>[4x]MASSNVTLSNDEVLRLVKDWNFTWSVVFLLITIVLQYGYPSRSMFVYVIKMFVLWLLWPASMALSIFCAVYPIDLASQIISGILAATSCAMWISYFVQSIRLFMRTGSWWSFNPESNCLLNVPIGGTTVVRPLVEDSTSVTAVVTDGYLKMAGMHFGACDFQRLPSEVTVAKPNVLIALKMIKRQAYGTNSGVAIYHRYKAGNYRRPPIIQDQELALLRA

The membrane (M) protein is the most abundant structural protein of coronaviruses including MERS-CoV, SARS-CoV, and SARS-CoV-2, and plays a central role in virus assembly through its interaction with various partner proteins. In coronaviruses, M protein is the only multispanning transmembrane structural protein and has been shown to interact with various partner proteins, including all viral structural proteins (S, M, E, and N) and some host factors involved in the interferon signaling pathway such as MAVS. Here, we present the first crystal structure of a betacoronavirus M protein from Pipistrellus bat coronavirus HKU5 (batCOV5-M), which is closely related to MERS-CoV, SARS-CoV, and SARS-CoV-2 M proteins. The batCOV5-M protein is closely related to MERS-M, and to a lesser extent, SARS-M and SARS2-M, sharing 95, 75 and 74% sequence homology, respectively.

After extensive crystallization trials and refinement, batCOV5-M crystallized in lipidic cubic phase (LCP) and the crystals diffracted to ∼3 Å resolution. The final batCOV5-M model was determined to 3.21 Å (batCOV5-Mxtal) and contained residues 13–199 of batCOV5-M, and the amino-terminus (12 residues) and the carboxy-terminus (21 residues) were not modeled due to weak electron densities. The batCOV5-Mxtal structure is organized as a homodimer, with each protomer containing a short amino-terminus, a three-helix transmembrane domain (TMD) and a cytosolic CTD consisting of an eight-stranded β-sandwich. The overall shape of the batCOV5-Mxtal dimer looks like a pair of pincers, with TMD as the “handle” and CTD as the “head” of the pincers. The two protomers form extensive TMD–TMD and CTD–CTD contacts with a buried area of ∼3,100 Å2 at the dimer interface, which accounts for ∼25% of the solvent-accessible surface area of each protomer, suggesting that the batCOV5-Mxtal dimer is a stable form. In the batCOV5-Mxtal structure, TM1 is placed almost in the sample plane as TM2/TM3, and the three helices of TMD resemble a capital letter “N,” while in SARS2-MAF the TMD helices form a more compact three-helix bundle. As a result, using TM2/TM3 as anchors, TM1 swings ∼40 degrees away from TM2 and CTD undergoes a rigid-body rotation of ∼30 degrees away from TMD during a transition from the “short” SARS2-MEM to the “long” batCOV5-Mxtal. Structural alignment yielded an all-Cα RMSD of 1.8 Å between batCOV5-Mxtal and SARS2-M-FabEM-long and an all-Cα RMSD of 1.6 Å between SARS2-MEM and SARS2-M-FabEM-short, while the major deviation came from flexible loops of these proteins. This result indicates that the structural organization is highly conserved in betacoronavirus M proteins, and the batCOV5-Mxtal structure represents the long conformation of M protein. In the second pattern, the N3C helix binds to a groove formed along the CTD dimer interface nearly vertical to the membrane plane.The BuVs, along with CuV and TuV belong to the genus Protoparvovirus, which prior the BuV discovery contained only animal (non-human) infecting viruses, and are classified as novel Primate protoparvovirus 1 species. The VP ORF encodes for two overlapping structural proteins, VP1 and VP2, sixty copies of which assemble their T = 1 icosahedral capsid in a predicted 1:10 ratio. The VP2 monomer extracted from the refined 60-mer capsids of the BuVs contained the core β-strands (βA–βI) and α-helix A (αA) observed in other parvoviruses and large loop insertions between these secondary structure elements. However, unlike the animal protoparvoviruses, the bufavirus capsid contain three separated protrusions surrounding the 3-fold axes, as has been reported for members of the Dependoparvovirus genus, human parvovirus B19, and the HBoVs.

Movie frame micrographs collected for these VLPs, at two different cryo-EM resources (West/Midwest Consortium for High-Resolution Cryo Electron Microscopy and SECM4) yielded capsid structures to 2.84, 3.79, and 3.25 Å resolution from 29,596, 7564, and 5234 particle images, respectively, for BuV1, BuV2, and BuV3. The BuV1 VP2 sequence and structure as well as capsid structure was compared to other protoparvoviruses with available 3D structures. The lower sequence identity of BuV1 to the other protoparvoviruses resulted in it possessing the most divergent surface loop structures compared to the other viruses. The largest of these conformational differences was at VR-VIII, although noticeable differences also occurred at other VRs, for example, VR-I, VR-III, VR-VI, and VR-VII. The BuV1 VR-VIII loop difference to the other protoparvovirues stemmed from a deletion of ~11 residues compared to the other viruses. This deletion removed the residues closest to the three-fold axes, resulting in three separate protrusions (also in BuV2 and BuV3) compared to the other protoparvoviruses that have a single pinwheel protrusion centered at this axis. At the 2-fold region, the depression was conserved while VR-IX adopted a different conformation; on the 2-fold wall, VR-VI was larger in BuV1 due to an 8-residue insertion. At the 2/5-fold wall, VR-VII of BuV1 had a two-residue deletion and was conformationally different. The melting temperature (Tms) of the BuV capsids determined by DSF were 64.9 ± 0.2 °C for BuV1, 77.3 ± 0.3 °C for BuV2, and 73.4 ± 0.2 °C for BuV3. A cladogram generated for BuV1 as well as the protoparvoviruses and human infecting parvoviruses compared based on the VP2 sequences places BuV1 between the animal and human viruses. Consistent with this observation, despite the higher (~10%) BuV1 VP2 sequence identity to the protoparvoviruses, the three separated protrusion 3-fold morphology of the BuVs resembled the human infecting viruses rather than the single pinwheel of the protoparvoviruses.

>[60x]SGVGHSTGNYNNRTEFYYHGDEVTIVCHSSRHIHLNMSESEEYKIYDTDRGPRFPTDQTLQGRDTINDSYHAQVETPWFLINPNSWGTWMNPADFQQLTTTCREVTLEHLDQTLDNIVIKTVSKQGSGAEETTQYNNDLTALLQVALDKSNQLPWVADNMYLDSLGYIPWRPCKLKQYSYHVNFWNTIDIISGPQQNQWQQVKKEIRWDDLQFTPIETTTEIDLLRTGDSWTSGPYKFNTKPTQLSYHWQSTRHTGSVHPTDPPNAIGQQGQNIRDINGWQWGDRSDPMSAATRVSNFHIGYSWPEWRIHYGSGGPAINPGAPFSQAPWSTDPQVRLTQGASEKAIFDYNHGDDDPAHRDQWWQNNLPITGQTNWAPKNAHQANLSSNVPSRQEFWTQDYHNTFGPFTAVDDVGIQYPWGAIWTKTPDTTHKPMMSAHAPFICKDGPPGQLLVKLAPNYTENLQTDGLGNNRIVTYATFWWTGKLILKGKLRLPRQFNLYNLPGRPRGTEAKKFLPNEIGHFELPFMPGRCMPNYTM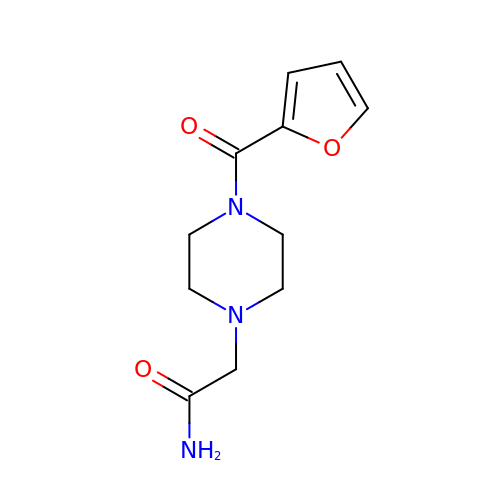2-[4-(furan-2-carbonyl)piperazin-1-yl]acetamide | C11 H15 N3 O3 | ZHALJTYSCWNFOY-UHFFFAOYSA-N>GSHDSGDKITATSSLKTPIVNRAITESEVLAAQKAWGEALVAISTTYDAKGKASAKALAEKVIDDAYGYQFGPVLFK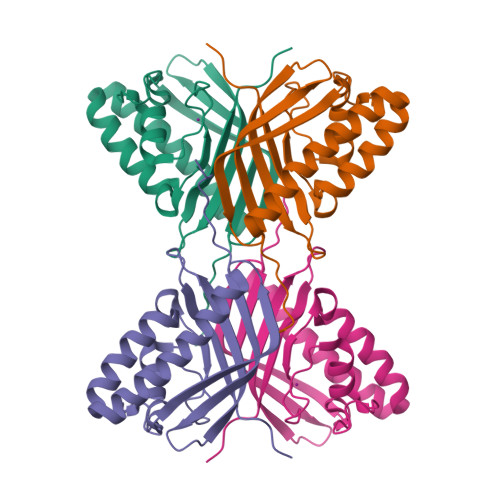PTLAISPRTFRTTRAGALAYFVGDDKAFPEDKGFALSSWRKVEIKNAAIFITGNTATTMGNVIITDKQGKATTVDKTWQFLKDDHGKLRIITHHSSLPYEQ[2x]>MQLFAAGVILFFLLALSGTIAGGLDVDSLQLPSEAAKFFHNDNSTNDDDSIGTRWAVLIAGSKGYHNYRHQADVCHMYQILRKGGVKDENIIVFMYDDIAYNESNPFPGIIINKPGGENVYKGVPKDYTGEDINNVNFLAAILGNKSAIIGGSGKVLDTSPNDHIFIYYANHGAPGKIGMPSKPYLYADDLVDTLKQKAATGTYKSMVFYVEACNAGSMFEGLLPEGTNIYAMAASNSTEGSWITYCPGTPDFPPEFDVCLGDLWSITFLEDCDAHNLRTETVHQQFELVKKKIAYASTVSQYGDIPISKDSLSVYMGTDPANDNRTFVDENSLRPPLKVIHQHDADLYHIWCKYNMAPEGSSKKIEAQKQLLELMSHRAHVDNSITLIGKLLFGVNKASKVLNTVRPVGQPLVDDWQCLKAMIRTFETHCGSLSEYGMKHTLSFANM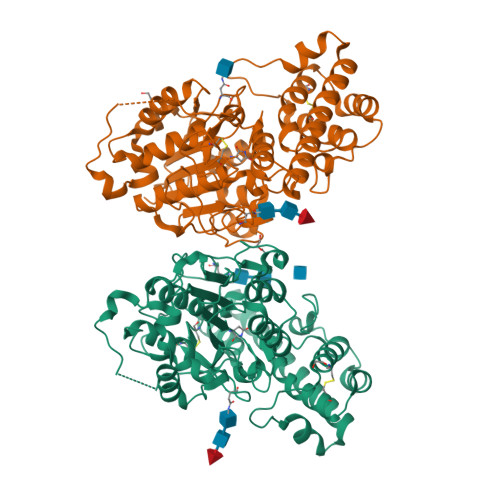CNAGIQKEQLAEAAAQACVTFPSNPYSSLAEGFSA[2x]[(2R,3S,4R,5R)-5-(6-amino-9H-purin-9-yl)-4-hydroxy-3-(phosphonooxy)oxolan-2-yl]methyl 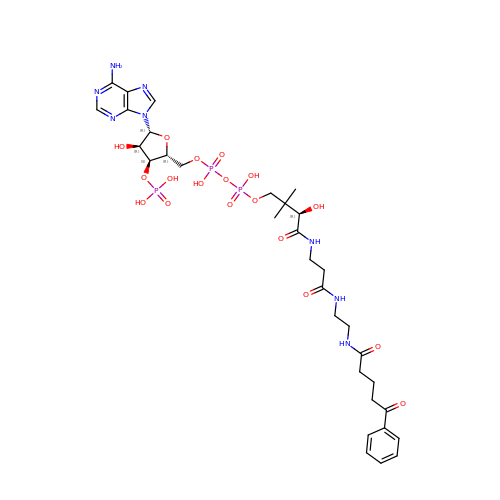(3R)-3-hydroxy-2,2-dimethyl-4-oxo-4-[(3-oxo-3-{[2-(5-oxo-5-phenylpentanamido)ethyl]amino}propyl)amino]butyl dihydrogen diphosphate | C32 H47 N8 O18 P3 | FIXBYTPINLXHIZ-GRBGHKMPSA-N> MVTIDSPVAGERFEAGKDINISATVKSKTPVSKVEFYNGDTLISSDTTAPYTAKITGAAVGAYNLKAVAVLSDGRRIESPVTPVLVKVIVKPTVKLTAPKSNVVAYGNEFLKITATASDSDGKISRVDFLVDGEVIGSDREAPYEYEWKAVEGNHEISVIAYDDDDA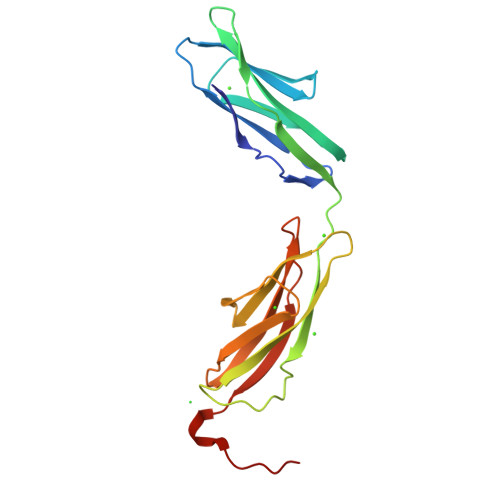ASTPDSVKIFVKQARLEHHHHHH> MIAVK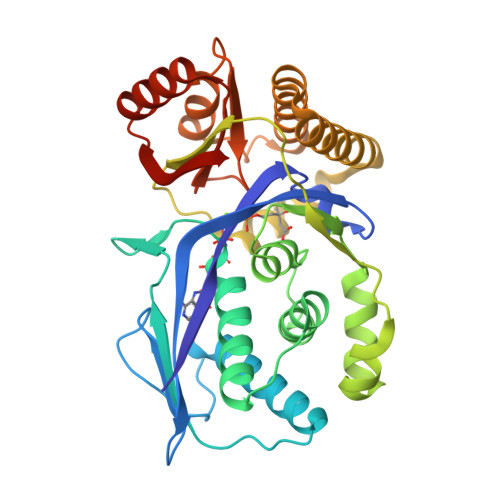TCGKLYWAGEYAILEPGQLALIKDIPIYMRAEIAFSDSYRIYSDMFDFAVDLRPNPDYSLIQETIALMGDFLAVRGQNLRPFSLAIYGKMEREGKKFGLGSSGSVVVLVVKALLALYNLSVDQNLLFKLTSAVLLKRGDNGSMGDLACIAAEDLVLYQSFDRQKVAAWLEEENLATVLERDWGFSISQVKPTLECDFLVGWTKEVAVSSHMVQQIKQNINQNFLTSSKETVVSLVEALEQGKSEKIIEQVEVASKLLEGLSTDIYTPLLRQLKEASQDLQAVAKSSGAGGGDCGIALSFDAQSTKTLKNRWADLGIELLYQERIGHDDKS>[2x]MREEQPHLATTWAARGWVEEEGIGSATLGRLVRAWPRRAAVVNKADILDEWADYDTLVPDYPLEIVPFAEHPLFLAAEPHQRQRVLTGMWIGYNERVIATEQLIAEPAFDLVMHGVFPGSDDPLIRKSVQQAIVDESFHTYMHMLAIDRTRELRKISERPPQPELVTYRRLRRVLADMPEQWERDIAVL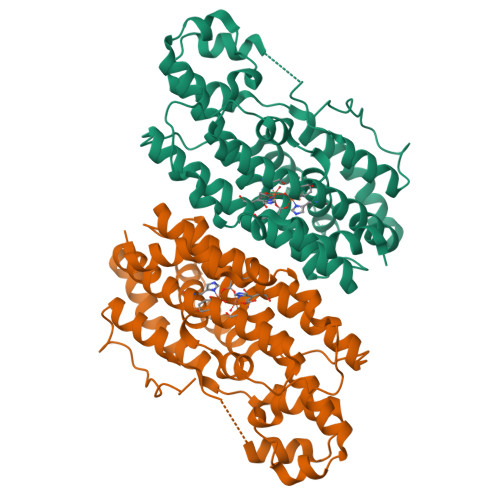VWGAVAETCINALLALLARDATIQPMHSLITTLHLRDETAHGSIVVEVVRELYARMNEQQRRALVRCLPIALEAFAEQDLSALLLELNAAGIRGAEEIVGDLRSTAGGTRLVRDFSGARKMVEQLGLDDAVDFDFPERPDWSPHTPR> PNFSGNWKIIRSENFEELLKVLGVNVMLRKIAVAAASKYAVEIKQEGDTFYIKVSTTVYTTEDNFKVGEEFEEQTVDGRPCKSLVKWESENKMVCEQKLLKGEGPKTSWTKELTNDGELIETMTAD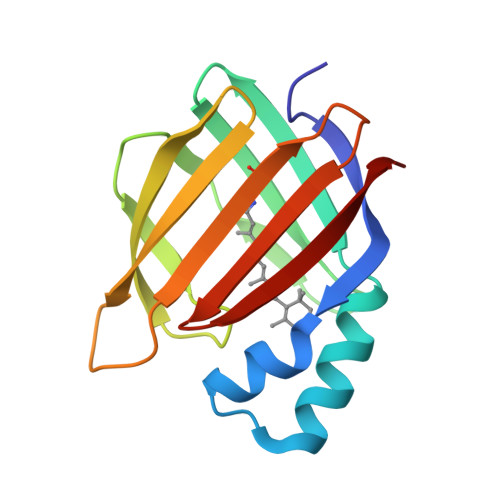DVVCTQVFVRE>RSVPSSTILIPVVVHVVYNNSAQNISDAQIISQIQVLNEDFRRMNADQANTPSAFANLAGNANIEFKLARRDPNGNTTNGITRTSTSTETFSMEMDNVKFSNLGGNNAWNTRRYLNIWVCNLGDDLLGYAQFPFEFQTKPNTDGVVIHYKHFGRDGSAESPYDKGRTATHEVGHWLDLRHIWGDDGGSCSGTDNIADTPNQGGYNEGCPSFPKTDHCTNTSPGVMFMNYMDYTYD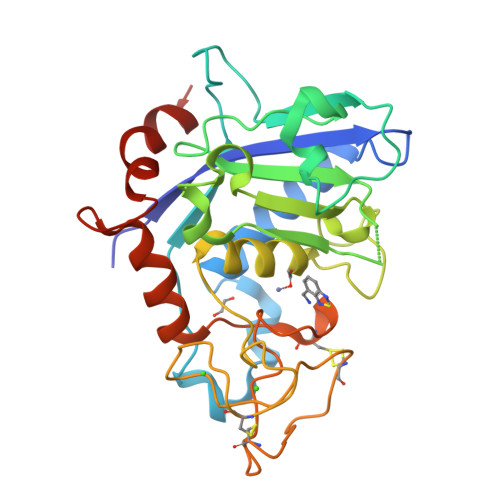ACMNLFTKGQVERMRSLFDTQTGIRREMQIYANELTNPLSFS[6x]>MGHHHHHHMKPYYVTTAIAYPNAAPHVGHAYEYIATDAIARFKRLDRYDVRFLTGTDEHGLKVAQAAAAAGVPTAALARRNSDVFQRMQEALNISFDRFIRTTDADHHEASKELWRRMSAAGDIYLDNYSGWYSVRDERFFVESETQLVDGTRLTVETGTPVTWTEEQTYFFRLSAYTDKLLAHYHANPDFIAPETRRNEVISFVSGGLDDLSISRTSFDWGVQVPEHPDHVMYVWVDALTNYLTGAGFPDTDSELFRRYWPADLHMIGKDIIRFHAVYWPAFLMSAGIELPRRIFAHGFLHNRGEKMSKSVGNIVDPVALAEALGVDQVRYFLLREVPFGQDGSYSDEAIVTRINTDLANELGNLAQRSLSMVAKNLDGRVPNPGEFADADAALLATADGLLERVRGHFDAQAMHLALEAIWLMLGDANKYFSVQQPWVLRKSESEADQARFRTTLYVTCEVVRIAALLIQPVMPESAGKILDLLGQAPNQRSFAAVGVRLTPGTALPPPTGVFPRYQPPQPPEGKRSHHHHHH[2x]

Methionyl-tRNA synthetase (MetRS) is a member of subclass Ia. MetRS is unique among the essential AARSs because it not only charges methionine to tRNA for elongation of translation, but also charges initiator tRNA to initialize translation. MetRS is considered to be one of the most promising drug targets in combatting bacterial pathogens, including MTB. The catalytic domain of MtMetRS spanning residues 1–115 (the N-terminal segment) and residues 226–292 (the C-terminal segment) has a typical α/β Rossmann fold.

Dh-MtMetRS with a double His tag was used for the crystallization of the apo-form enzyme, whereas N-terminally His-tagged MtMetRS was used for the crystallization of the Met-AMP-bound enzyme. The crystals of F-state MtMetRS diffracted X-rays to 1.9 Å resolution, belonged to space group P1 and contained two copies of MtMetRS in the asymmetric unit. In F-state MtMetRS the entire α2 helix (residues 50–62) connecting β2 and α3 disappeared from the electron-density map, suggesting high flexibility of this region. The KMSKS loop forming the distal end of the AMP pocket was completely missing in the F-state enzyme. Ile10 and Tyr12, which constitute the upper wall of the methionine cavity, push into the methionine pocket (Cα displacements of 2.6 and 5.1 Å) and hence the pocket essentially collapses. Collectively, our crystallographic investigations revealed a previously unobserved active site in F-state MtMetRS which appears to be nonproductive. We illustrate in Figs. 4(a) and 4(b) that while the active site is well ordered in P-state MtMetRS, the methionine pocket collapses and the AMP pocket shrinks significantly in the F-state enzyme. The cavity of the active site has a volume of 2186 Å3 in the presence of Met-AMP; in contrast, it reduced to 360 Å3 in the absence of the ligand. In sharp contrast, we found that F-state MtMetRS is characterized by a completely collapsed methionine pocket, a nonexistent AP and a severely reduced groove for adenosine. The HVGH motif adopting the rare β-turn conformation in the apo structure is not involved in crystal contacts, suggesting that the observed conformation does not result from crystal-packing artifacts. The unusual F-state structure of MtMetRS observed here reflects the intrinsic flexibility of the catalytic core, which is unique among the characterized MetRSs.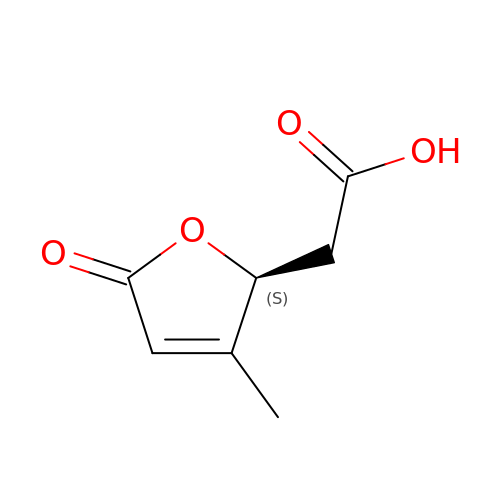[(2S)-3-methyl-5-oxo-2,5-dihydrofuran-2-yl]acetic acid | C7 H8 O4 | GXEVIPDDAUJTCF-YFKPBYRVSA-N> CDIHVLWEWKCFEEL;>EVVKFMDVYQRSYCHPIETLVDIFQEYPDEIEYIFKPSCVPLMRCGGCCNDEGLECVPTEESNITMQIMRIKPHQGQHIGEMSFLQHNKCECRPK[2x]

In the present work, we focus on a class of monocyclic disulfide‐containing 19 amino acid peptides targeting the Vascular Endothelial Growth Factor‐A, the main pro‐angiogenic factor in Human. We proposed to use this peptide as a model to rationalize the thermodynamics of α‐helix stabilization by an i to i+4 lactam bridge. Around 950 Å2 of accessible surface area (ASA) was buried at the peptide‐VEGF interface, that overlapped with the VEGF receptor 1 domain 2 (VEGFR1‐d2)‐binding site. Although only lactam‐bridged ExxxK, DxxxK and KxxxD induced the formation of stable helix in the unbound state, all peptides of the series were helically folded when bound to VEGF.

Constraints caused by the lactam bridges and by the binding of the macro‐cyclized peptide to the VEGF site also made the α‐helices non‐canonical: in each of the four peptides, the residues P8‐11 folded into a 310‐helix characterized by a H‐bond between Glu P8 O and Cys P11 HN. The helix of peptide 4 c (KxxxE) was longer (residues P8 to P14) with a H‐bond network similar to peptide 2 c. In contrast, the helix of peptide 4 c was poorly defined in the electronic density (RSCC=0.76). In the 4 c peptide, the lactam bridge cyclization forced Lys P14 to rotate along phi angle (ϕLys,P14=−47°), which prevented any folding of the P15 residue into the helix. Indeed, crystal structure and NMR data evidenced that the C‐terminus part of the 4 c helix was poorly structured, making it the most dynamic among the bicyclic peptides. Although P10 and P14 residues were in standard rotamer conformation, the constraints due to the lactam bridge destabilized the helix fold and acted as helix breaker at the P15 residue. On the contrary, the monocyclic peptides 1, 2, 3 and 4, and the peptide 4 c had little secondary structure: they displayed a weak maximum at 190 nm, a negative minimum at 204–205 nm followed by a positive slope reaching zero at around 225 nm and forming a small positive peak around 228 nm.> MRRLLFLSLAGLWLFSPAAAAQLPGLISQPLAGGGQSWSLSVQTLVFITSLTFLPAILLMMTSFTRIIIVFGLLRNALGTPSAPPNQVLLGLALFLTFFIMSPVIDKIYVDAYQPFSEQKISMQEALDKGAQPLRAFMLRQTREADLALFARLANSGPLQGPEAVPMRILLPAYVTSELKTAFQIGFTIFIPFLIIDLVIASVLMALGMMMV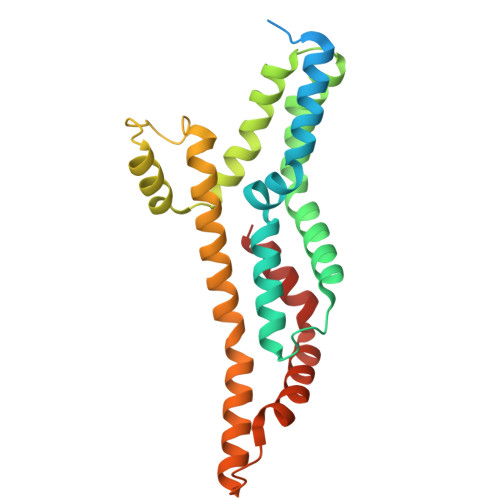PPATIALPFKLMLFVLVDGWQLLMGSLAQSFYS> LTFLEY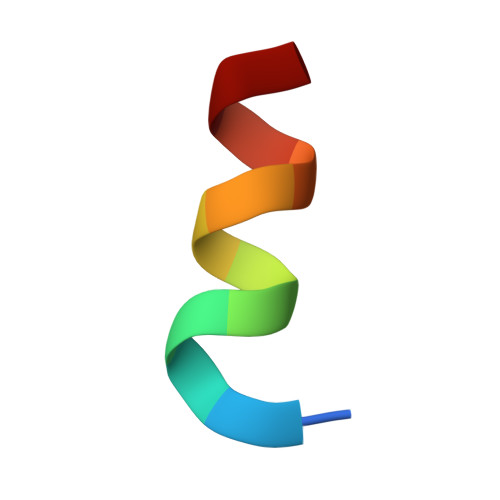WAQLMQ> MSKQFVRSAKNMMKGYSSTQVLVRDATANDSRTPSIDTLDDLAQRSYDSVDFFEIMDMLDKRLNDKGKYWRHVAKSLTVLDYLVRFGSENCVLWCRENFYVIKTLREFRHENESGFDEGQIIRVKAKELVSLLNDEERLREERSMNTRNRRANRAA

Clathrin-mediated endocytosis is essential for protein retrieval during neurotransmission and receptor recycling. Accumulation of the adapter proteins at the plasma membrane initiates the endocytic event and contributes to membrane bending. Complex formation has been observed between the ENTH domain of epsin and the ANTH domain of Sla2, the yeast homolog of human huntingtin interacting protein 1 related (Hip1R). Epsin and the phospholipid PIP2 are essential for clathrin-mediated endocytosis, and we show how assemblies are formed between the ENTH domain of epsin and the ANTH domain of Sla2 in fungi.

The Ent1 and Ent2 ENTH domains (ENTH1 and ENTH2) from S. cerevisiae as well as an ENTH domain of homologous epsin from C. thermophilum bind up to two PIP2 molecules per domain. We tested complex formation between the S. cerevisiae ENTH2 domain and the ANTH domain of Sla2 to verify the assembly relevant to the ENTH2/PIP2 crystal structure. Indeed, an assembly with a stoichiometry of 8:8:24 ± 3 for ENTH2/ANTHSla2/PIP2 is formed, similar to the ENTH1 complex and ENTH/ANTHSla2 complex of C. thermophilum. When equal amounts of S. cerevisiae ENTH1 and ENTH2 are mixed together with ANTHSla2 and measured by native MS, a complex containing equal amounts of ENTH1 and ENTH2 is formed, showing no preference for either isoform and highlighting the possibility to recruit different epsins into a complex with Sla2.> MADVINVSVNLEAFSQAISAIQALRSSVSRVFDCLKDGMRNKETLEGREKAFIAHFQDNLHSVNRDLNELERLSNLVGKPSENHPLHNSGLLSLDPVQDKTPLYSQLLQAYKWSNKLQYHAGLASGLLNQQSLKRSANQMGVSAKRRPKAQPTTLVLPPQYVDDVISRIDRMFPEMSIHLSRPNGTSAMLLVTLGKVLKVIVVMRSLFIDRTIVKGYNENVYTEDGKLDIWSKSNYQVFQKVTDHATTALLHYQLPQMPDVVVRSFMTWLRSYIKLFQA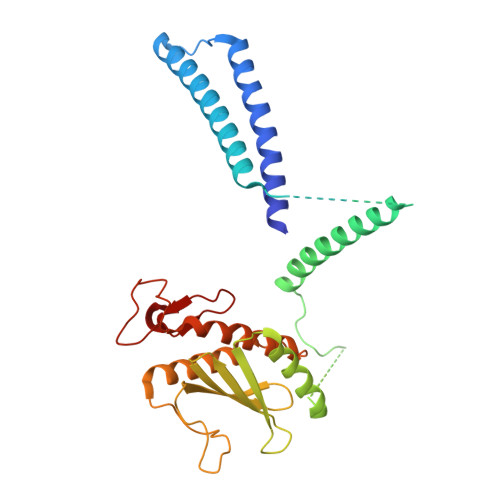PCQRCGKFLQDGLPPTWRDFRTLEAFHDTCRQ>[2x]MNLKALPAIEGDHNLKNYEETYRHFDWAEAEKHFSWHETGKLNAAYEAIDRHAESFRKNKVALYYKDAKRDEKYTFKEMKEESNRAGNVLRRYGNVEKGDRVFIFMPRSPELYFIMLGAIKIGAIAGPLFEAFMEGAVKDRLENSEAKVVVTTPELLERIPVDKLPHLQHVFVVGGEAESGTNIINYDEAAKQESTRLDIEWMDKKDGFLLHYTSGSTGTPKGVLHVHEAMIQQYQTGKWVLDLKEEDIYWCTADPGWVTGTVYGIFAPWLNGATNVIVGGRFSPESWYGTIEQLGVNVWYSAPTAFRMLMGAGDEMAAKYDLTSLRHVLSVGEPLNPEVIRWGHKVFNKRIHDTWWMTETGSQLICNYPCMDIKPGSMGKPIPGVEAAIVDNQGNELPPYRMGNLAIKKGWPSMMHTIWNNPEKYESYFMPGGWYVSGDSAYMDEEGYFWFQGRVDDVIMTSGERVGPFEVESKLVEHPAIAEAGVIGKPDPVRGEIIKAFIALREGFEPSDKLKEEIRLFVKQGLAAHAAPREIEFKDKLPKTRSGKIMRRVLKAWELNLPAGDLSTMED

Acetyl-CoA synthetase (Acs) generates acetyl-coenzyme A (Ac-CoA) but its excessive activity can deplete ATP and lead to a growth arrest. To prevent this, Acs is regulated through Ac-CoA-dependent feedback inhibition executed by Ac-CoA-dependent acetyltransferases such as AcuA in Bacillus subtilis. AcuA acetylates the catalytic lysine of AcsA turning the synthetase inactive. Acs enzymes consists of two consecutively operating modules, a C-terminal domain (CTD) catalyzing the first and a N-terminal domain (NTD) for the second reaction step.

Initial three-dimensional (3D) classification (T = 4) of 1,194,314 selected particles using AlphaFold-predicted AcsA dimer as starting model yielded two distinct states. After multiple rounds of processing, those two states were turned out to be AcsA homodimer and AcsA-AcuA complex, determined at 2.89 Å and 2.93 Å resolution, respectively. MP analysis of AcsA alone (i.e., 37.5 nM) resulted in detection of a monomer (71 kDa) and a dimer (140 kDa).Human enteropeptidase (hEP), also known as enterokinase, is an essential enzyme in food digestion and is localized at the brush border of the duodenal and jejunal mucosa. Activated hEP can stimulate the conversion of trypsinogen to trypsin via cleavage of a specific trypsinogen activation peptide, namely Asp-Asp-Asp-Asp-Lys (DDDDK), which is highly conserved in vertebrates. However, the mechanism of hEP activation remains to be established. hEP contains a multi-domain heavy chain and a catalytic light chain, linked by a disulfide bond. The functions of these domains and motifs may be involved in protein anchoring, macromolecular substrate recognition and inhibitor specificity. The light chain is homologous to trypsin-like serine proteinases with a typical Asp-His-Ser (D-H-S) catalytic triad responsible for peptidase activity.

Since the SEA domain has been shown to be dispensable for the enzymatic activity, a further truncated hEP including only residues 182–1019, i.e., also leaving out the SEA domain, was used for further high-resolution structural analysis. The resulting purified hEP was a heavily glycosylated single-chain zymogen with a molecular weight (>130 kDa) higher than that theoretically predicted of the amino acids alone (95 kDa). An enzymatic activity assay performed in vitro confirmed its inactive state with no detectable substrate cleavage as previously described, and the hEP became active upon cleavage by trypsin into two chains. Cryo-EM single-particle analysis of this inactive hEP yielded a cryo-EM reconstruction at 3.8 Å resolution, with the resolution of the core region reaching 2.7 Å, allowing explicit visualization of side-chain density of most residues except for those of surface loops L1, L2, and LD in the peptidase domain. The overall architecture of this inactive hEP was the same as that containing the SEA domain (residues 48–1019), showing a clamp shape adopted by the heavy chain with the light chain in the center. The LDLR, CUB, and MAM (LCM) domains were observed to protrude from the remainder of the hEP-core region, which containing the CUB2, LDLR2, and SRCR domains of the heavy chain and the peptidase domain of the light chain, resulting in lower local resolution likely due to high flexibility of the LCM relative to the core region. In addition to the disulfide bond (Cys772-Cys896) between the light and heavy chains, the CUB2 and SRCR domains stabilized the peptidase domain by forming hydrogen bonds between Glu581 and Arg871, and between Ser771 and Gln893. The CUB2 and SRCR domains were interconnected by the LDLR2 domain, and clamped the peptidase domain with a total interaction surface of 1163.2 Å2. Additional density for glycans was observed at all nine N-glycosylation sites in the inactive hEP-core region, suggesting a near-physiological state of our inactive hEP structure.

> ELPTDCGGPFELWEPNTTFSSTNFPNSYPNLAFCVWILNAQKGKNIQLHFQEFDLENINDVVEIRDGEEADSLLLAVYTGPGPVKDVFSTTNRMTVLLITNDVLARGGFKANFTTGYHLGIPEPCKADHFQCKNGECVPLVNLCDGHLHCEDGSDEADCVRFFNGTTNNNGLVRFRIQSIWHTACAENWTTQISNDVCQLLGLGSGNSSKPIFPTDGGPFVKLNTAPDGHLILTPSQQCLQDSLIRLQCNHKSCGKKLAAQDITPKIVGGSNAKEGAWPWVVGLYYGGRLLCGASLVSSDWLVSAAHCVYGRNLEPSKWTAILGLHMKSNLTSPQTVPRLIDEIVINPHYNRRRKDNDIAMMHLEFKVNYTDYIQPICLPEENQVFPPGRNCSIAGWGTVVYQGTTANILQEADVPLLSNERCQQQMPEYNITENMICAGYEEGGIDSCQGDSGGPLMCQENNRWFLAGVTSFGYKCALPNRPGVYARVSRFTEWIQSFLH> MSVVSQVILQADDQLRYPTSGELKGIQAFLTTGAQRIRIAETLAENEKKIVDQAQKQLFKKHPEYRAPGGNAYGQRQYNQCLRDYGWYLRLVTYGVLAGNKEPIETTGLIGVKEMYNSLNVPVPG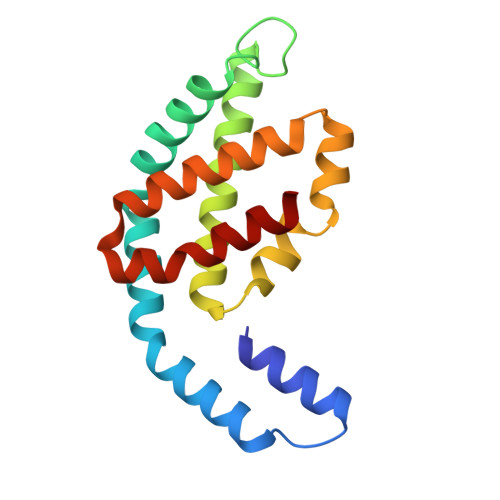MVDAVTVLKDAALGLLSAEDANETAPYFDYIIQFMS The Lon protease is a AAA+ protein found in prokaryotes, archaea, and eukaryotic organelles. Lon is involved in cellular protein homeostasis by degrading damaged or misfolded abnormal proteins, which prevents these unwanted protein species from forming toxic aggregates. Lon is known to form a homohexamer; each protomer is composed of multiple domains, including an N-terminal substrate-binding globular domain (NGD), a long-helix domain (LH), a three-helix bundle (3H), a AAA+ ATPase module, and a protease domain. We show here, using cryo-electron microscopy (cryo-EM), that the activation process of the Lon AAA+ protease may involve a pentameric assembly and a substrate-dependent incorporation of the sixth protomer to form the substrate-pore-loop contacts seen in the translocating state.

To provide a comparative context, we also examined wild-type MtaLon in two states: without any nucleotide (MtaLon-Apo) and incubated with 5 mM ADP (MtaLon:ADP). Additionally, our cryo-EM structures of a series of spiral subcomplex oligomers of Lon determined by 3D reconstructions suggest a sequential pathway for the construction of the THT. In the proposed pathway, the THT is formed by sequential incorporation of the protomers, beginning with Ob1 and progressing in the clockwise direction through Ob5, and completed by the incorporation of Ac6*, whose binding mode is dependent on the substrate.

>MRLELPVIPLRNTVILPHTTTPVDVGRAKSKRAVEEAMGADRLIFLVAQRDPEVDDPAPDDLYTWGVQAVVKQAMRLPDGTLQVMVEARARAQVTDYIPGPYLRARGEVFSEIFPIDEAVVRVLVEELKEAFEKYVANHKSLRLDRYQLEAVKGTSDPAMLADTIAYHATWTVAEKQEILELTDLEARLKKVLGLLSRDLERFELDKRVAQRVKEQMDTNQREYYLREQMKAIQKELGGEDGLSDLEALRKKIEEVGMPEAVKTKALKELDRLERMQQGSPEATVARTYLDWLTEVPWSKADPEVLDINHTRQVLDEDHYGLKDVKERILEYLAVRQLTQGLDVRNKAPILVLVGPPGVGKTSLGRSIARSMNRKFHRISLGGVRDEAEIRGHRRTYIGAMPGKLIHAMKQVGVINPVILLDEIDKMSSDWRGDPASAMLEVLDPEQNNTFTDHYLDVPYDLSKVFFITTANTLQTIPRPLLDRMEVIEIPGYTNMEKQAIARQYLWPKQVRESGMEGRIEVTDAAILRVISEYTREAGVRGLERELGKIARKGAKFWLEGAWEGLRTIDASDIPTYLGIPRYRPDKAETEPQVGTAQGLAWTPVGGTLLTIEVAAVPGSGKLSLTGQLGEVMKESAQAALTYLRAHTQDYGLPEDFYNKVDLHVHVPDGATPKDGPSAGITMATAIASALSRRPARMDIAMTGEVSLRGKVMPIGGVKEKLLAAHQAGIHKIVLPKDNEAQLEELPKEVLEGLEIKLVEDVGEVLEYLLLPEPTMPPVVQPSDNRQQPGAGA[4x]> SVKILVVEDNHVNQEVIKRMLNLEGIENIELACDGQEAFDKVKELTSKGENYNMIFMD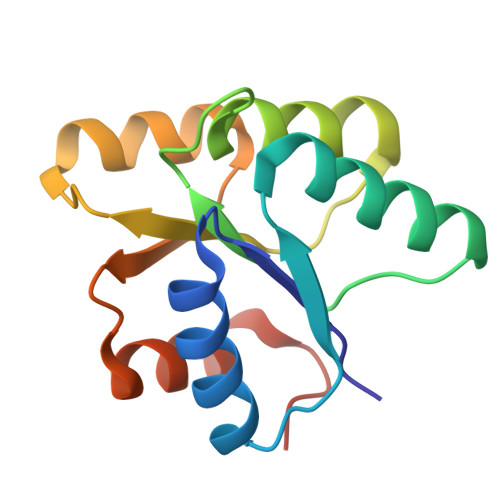VQMPKVDGLLSTKMIRRDLGYTSPIVALTAFADDSNIKECLESGMNGFLSKPIKRPKLKTILTEFCAAYQGKKNNK>SSVDGASGAGQLVPEVNASDPLAMDPVAGSSTAVATAGQVNPIDPWIINNFVQAPQGEFTISPNNTPGDVLFDLSLGP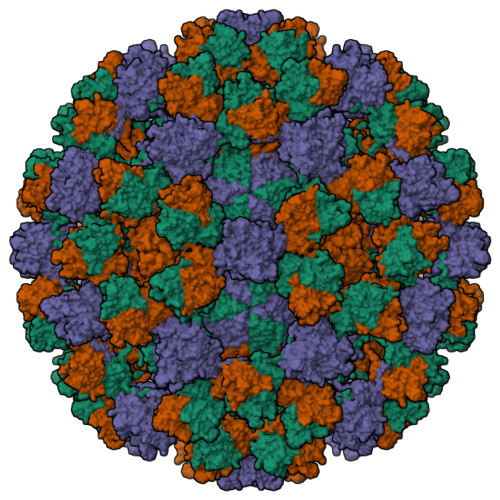HLNPFLLHLSQMYNGWVGNMRVRIMLAGNAFTAGKIIVSCIPPGFGSHNLTIAQATLFPHVIADVRTLDPIEVPLEDVRNVLFHNNDRNQQTMRLVCMLYTPLRTGGGTGDSFVVAGRVMTCPSPDFNFLFLVPAAAAAARMVDLPVIQPRLCTHARWPAPVYGLLVDPSLPSNPQWQNGRVHVDGTLLGTTPISGSWVSCFAAEAAYEFQSGTGEVATFTLIEQDGSAYVPGDRAAPLGYPDFSGQLEIEVQTETTKTGDKLKVTTFEMILGPTTNADQAPYQGRVFASVTAAASLDLVDGRVRAVPRSIYGFQDTIPEYNDGLLVPLAPPIGPFLPGEVLLRFRTYMRQIDTADAAAEAIDCALPQEFVSWFASNAFTVQSEALLLRYRNTLTGQLLFECKLYNEGYIALSYSGSGPLTFPTDGIFEVVSWVPRLYQLASVGSLATGRMLK[3x]> MIEKSQACHDSLLDSVGQTPMVQLHQLFPKHEVFAKLEYMNPGGSMKDRPAKYIIEHGIKHGLITENTHLIESTSGNLGIALAMIAKIKGLKLTCVVDPKISPTNLKIIKSYGANVEM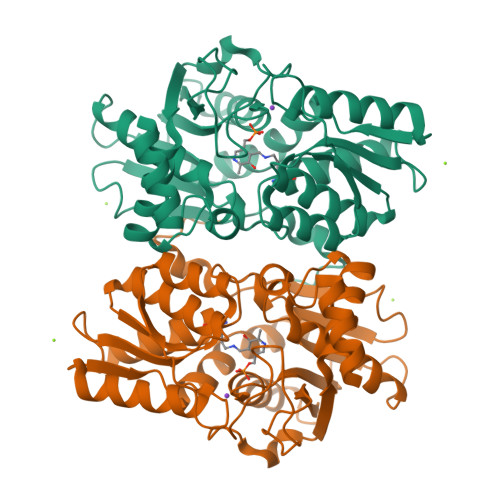VEEPDAHGGYLMTRIAKVQELLATIDDAYWINQFANELNWQSHYHGAGTEIVETIKQPIDYFVAPVGTTGSIMGMSRKIKEVHPNAQIVAVDAKGSVIFGDKPINRELPGIGASRVPEILNRSEINQVIHVDDYQSALGCRKLIDYEGIFAGGSTGSIIAAIEQLITSIEEGATIVTILPDRGDRYLDLVYSDTWLEKMKSRQGVKSE> MVTSKPINARPLPAGLTASQQWT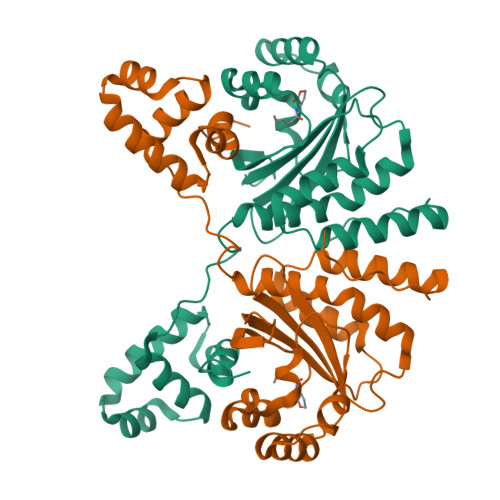LLEWIHMAGHIETEGELKAFLDNILSQAPSDRIILVLGRLNNQNQIQRMEKVLNVSYPSDWLNQYSQENFAQHDPIMRIHLGQGPVIWEERFSRAKGSEEKRFIAEASSNGMGSGITFSAASDRNNVGSILSIGGKEPGRNAALVAMLNCLTPHLHQAAVRIANLPPASPSNMPLSQREYDIFHWMSRGKTNWEIATILNISERTVKFHVANVIRKLNANNRTHAIVLGMHLAMTPRELVNG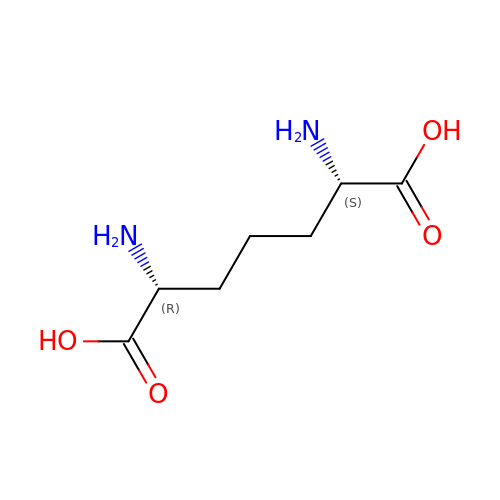2,6-DIAMINOPIMELIC ACID | C7 H14 N2 O4 | GMKMEZVLHJARHF-SYDPRGILSA-N>GSGEADMDFLRNLFSQTLSLGSQKERLLDELTLEGVARYMQSERCRRVICLVGAGISTSAGIPDFRSPSTGLYDNLEKYHLPYPEAIFEISYFKKHPEPFFALAKELYPGQFKPTICHYFMRLLKDKGLLLRCYTQNIDTLERIAGLEQEDLVEAHGTFYTSHCVSASCRHEYPLSWMKEKIFSEVTPKCEDCQSLVKPDIVFFGESPPARFFSCMQSDFLKVDLLLVMGTSLQVQPFASLISKAPLSTPRLLINKEKAGQSDPFLGMIMGLGGGMDFDSKKAYRDVAWLGECDQ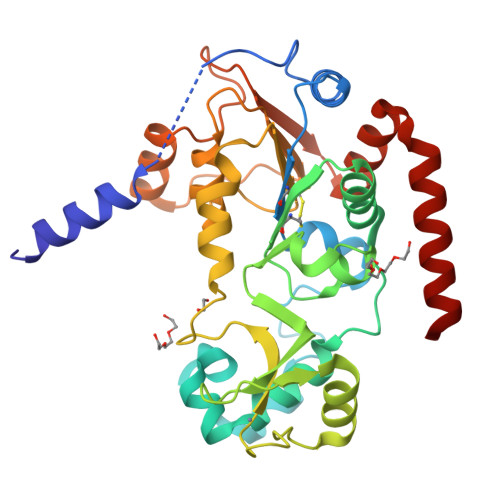GCLALAELLGWKKELEDLVRREHASIDAQS[3x]> MDRINESHQRFLQALMSHGIMEGSAVRALHRHCCELHKVHYMHDKLDDFVGVLNRHLQPLFMTIEKG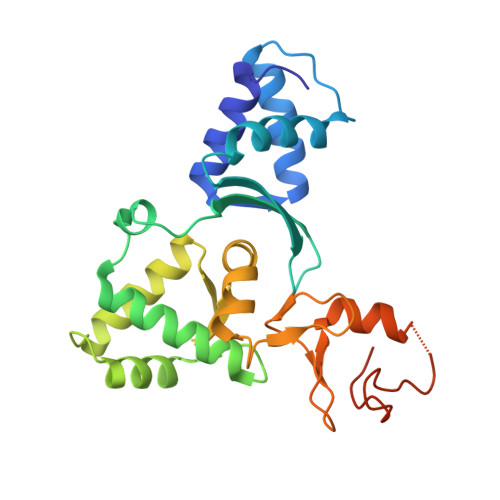VGEEDGLTYYALVNRVENDITKMASDYAENELELFRKTMELIILSDNGFATSISILNLADELQSKKMKKKEVEQLLQSFVQEKWLIGRNGEYTLHTRCIMELEHYIRNTYQDVAKICNVCRKVAIQSQLCENCGIPLHLQCAGKYFHGKANPTCPNCNESWPHEIPDLNQVSSQGPSHSQ> GAMGSKISNIFEDVEFCVMSGTDSQPKPDLENRIAEFGGYIVQNPGPDTYCVIAGSENIRVKNIILSNKHDVVKPAWLLECFKTKSFVPWQPRFMIHMCPSTKEH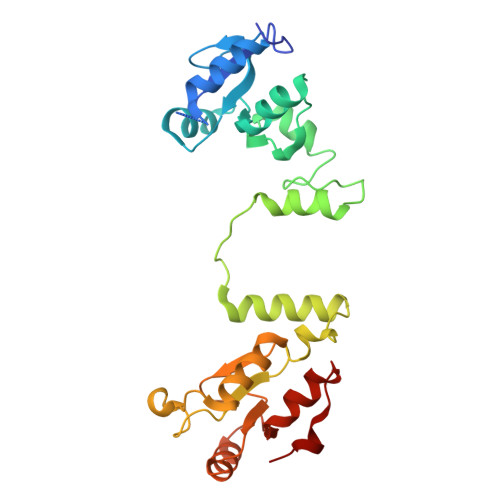FAREYDCYGDSYFIDTDLNQLKEVFSGIKNSNEQTPEEMASLIADLEYRYSWDCSPLSMFRRHTVYLDSYAVINDLSTKNEGTRLAIKALELRFHGAKVVSCLAEGVSHVIIGEDHSRVADFKAFRRTFKRKFKILKESWVTDSIDKCELQEENQYLI>[2x]MGRIKNKQFAVIGLGKFGGSICKELHRMGHEVLAVDINEEKVNAYASYATHAVIANATEENELLSLGIRNFEYVIVAIGANIQASTLTTLLLKELDIPNIWVKAQNYYHHKVLEKIG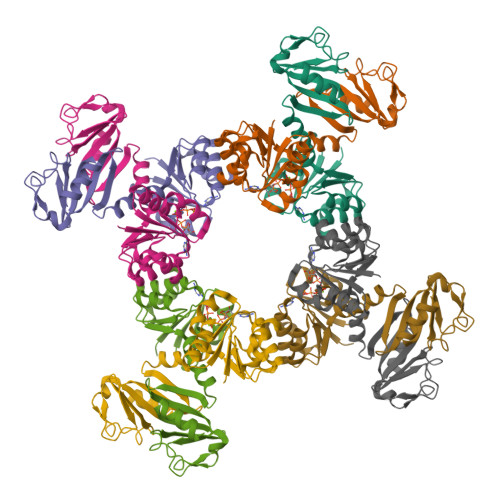ADRIIHPEKDMGVKIAQSLSDENVLNYIDLSDEYSIVELLATRKLDSKSIIDLNVRAKYGCTILAIKHHGDICLSPAPEDIIREQDCLVIMGHKKDIKRFENEGM> MLYVEILGNLPEMARDEVKAMLELGGGEIIGQDYLFLKVDAGEKAFPFLDRLGLAHEYGLLLVEADSVEELLQKAGEVEWPIKGAFKVDTETMANCRHDVLDLPRKLGAVIHAQG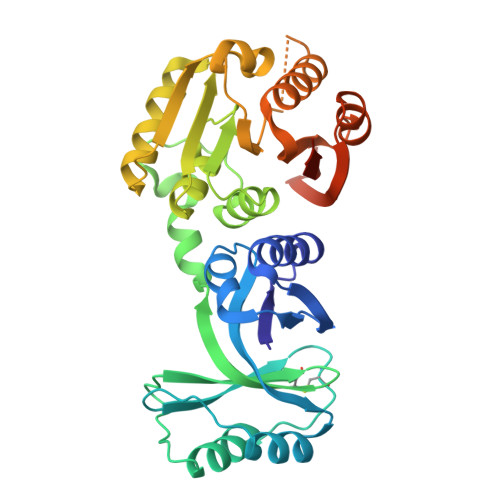FRVNLSKPDTVVRVYCGERLYAGIRLRYFDPKDFEKRKAHHRPFFRPISLHPRVSRALVNLTKATREILDPFMGAGGILIEAGLLGLRVYGVDIRPEMVEGAETNLKHYGVRDYTLKLGDATRLEDLFPDKKFEAVATDPPYGTAATLAGRKRDELYRKALRSIYNVLEDGGRLAIAFPTDFNGKAEAEAVGFRTLGRYYQRVHKSLERYFYVFEKLEVLFQGPSHHHHHH> MKKVEYWVKIPFGPIHPGLEEPEKFIITLDGERIVNVDVKLGYNLRGVQWIGMRRNYVQIMYLAERMCGICSFSHNHTYVRAVEEMAGIEVPERAEYIRVIVGELERIHSHLLNLGVVGHDIGYDTVLHLTWLARERVMDVLEAVSGNRVNYSMVTIGGVRRDIGEKQKRLILDMIKYYREVLPQIEDVFLHDSTIEARLRDVAVVPKKLAIEMGAVGPTARGSGIKEDSRWSEQLGVYPDLGIKPVTPEDVTGEKARGDVYDRMAVRIGELWMSLDLLEHALDQMPEGKIKTFPKDNILVAKLKLLGDGEGIGRYEAPRGELVHYVRGQKGRDGPVRWKPREPTFPNLFTIAKALEGNELADLVVAIASIDPCL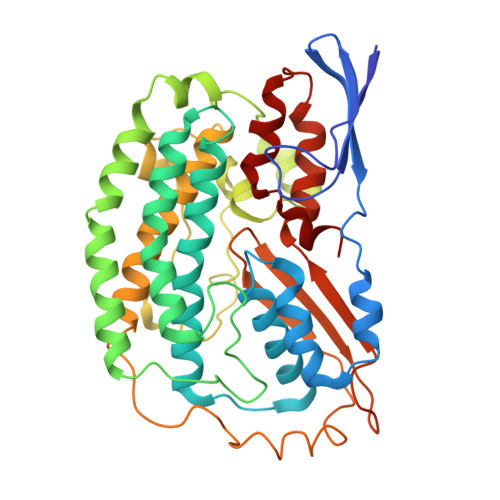SCTDR> MAHHHHHHHHHHGSTSGSGEQKLISEEDLGSTSGSGDYKDDDDKLTSLYKKAGLENLYFQGMESEMLQSPLLGLGEEDEADLTDWNLPLAFMKKRHCEKIEGSKSLAQSWRMKDRMKTVSVALVLCLNVGVDPPDVVKTTPCARLECWIDPLSMGPQKALETIGANLQKQYENWQPRARYKQSLDPTVDEVKKLCTSLRRNAKEERVLFHYNGHGVPRPTVNGEVWVFNKNYTQYIPLSIYDLQTWMGSPSIFVYDCSNAGLIVKSFKQFALQREQELEVAAINPNHPLAQMPLPPSMKNCIQLAACEATELLPMIPDLPADLFTSCLTTPIKIALRWFCMQKCVSLVPGVTLDLIEKIPGRLNDRRTPLGELNWIFTAITDTIAWNVLPRDLFQKLFRQDLLVASLFRNFLLAERIMRSYNCTPVSSPRLPPTYMHAMWQAWDLAVDICLSQLPTIIEEGTAFRHSPFFAEQLTAFQVWLTMGVENRNPPEQLPIVLQVLLSQVHRLRALDLLGRFLDLGPWAVSLALSVGIFPYVLKLLQSSARELRPLLVFIWAKILAVDSSCQADLVKDNGHKYFLSVLADPYMPAEHRTMTAFILAVIVNSYHTGQEACLQGNLIAICLEQLNDPHPLLRQWVAICLGRIWQNFDSARWCGVRDSAHEKLYSLLSDPIPEVRCAAVFALGTFVGNSAERTDHSTTIDHNVAMMLAQLVSDGSPMVRKELVVALSHLVVQYESNFCTVALQFIEEEKNYALPSPATTEGGSLTPVRDSPCTPRLRSVSSYGNIRAVATARSLNKSLQNLSLTEESGGAVAFSPGNLSTSSSASSTLGSPENEEHILSFETIDKMRRASSYSSLNSLIGVSFNSVYTQIWRVLLHLAADPYPEVSDVAMKVLNSIAYKATVNARPQRVLDTSSLTQSAPASPTNKGVHIHQAGGSPPASSTSSSSLTNDVAKQPVSRDLPSGRPGTTGPAGAQYTPHSHQFPRTRKMFDKGPEQTADDA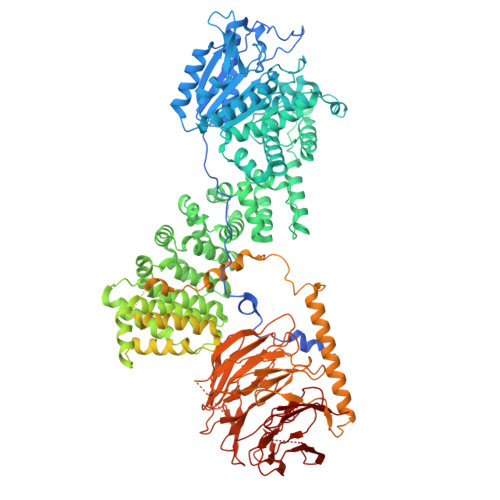DDAAGHKSFISATVQTGFCDWSARYFAQPVMKIPEEHDLESQIRKEREWRFLRNSRVRRQAQQVIQKGITRLDDQIFLNRNPGVPSVVKFHPFTPCIAVADKDSICFWDWEKGEKLDYFHNGNPRYTRVTAMEYLNGQDCSLLLTATDDGAIRVWKNFADLEKNPEMVTAWQGLSDMLPTTRGAGMVVDWEQETGLLMSSGDVRIVRIWDTDREMKVQDIPTGADSCVTSLSCDSHRSLIVAGLGDGSIRVYDRRMALSECRVMTYREHTAWVVKASLQKRPDGHIVSVSVNGDVRIFDPRMPESVNVLQIVKGLTALDIHPQADLIACGSVNQFTAIYNSSGELINNIKYYDGFMGQRVGAISCLAFHPHWPHLAVGSNDYYISVYSVEKRVR> DLT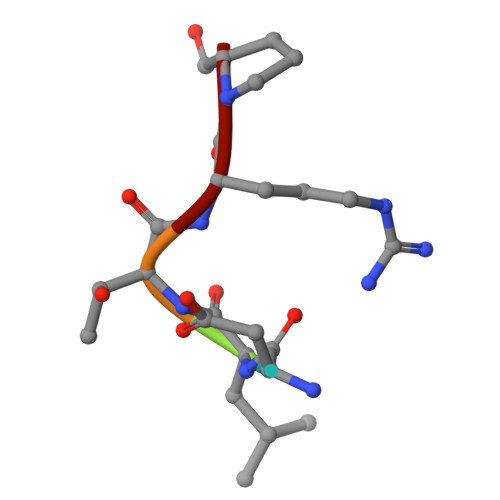RP> GPLGSPEFMTLEEVRGQDTVPESTARMQGAGKALHELLLSAQRQGCLTAGVYESAKVLNVDPDNVTFCVLAAGEEDEGDIALQIHFTLIQAFCCENDIDIVRVGDVQRLAAIVGAGEEAGA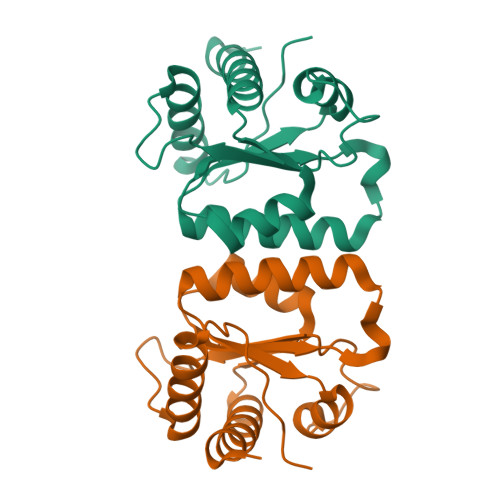PGDLHCILISNPNEDAWKDPALEKLSLFCEESRSVNDWVPSITLPE> GGMTTMTVHTMGVHYKWQIPEVLRQQLWLAHNLREDLVSLQLAYDDDLKAIWSSYPDVAQAEDTMAAAEADAVALSERVKQARIEARSKKISTELTQQLRDAKKRLKDARQARRDAIAVVKDDAAERRKARSDQLAADQKALYGQYCRDGDLYWASFNTVLDHHKTAVKRIAAQRASGKPATLRHHRFDGSGTIAVQLQRQAGAPPRTPMVLADEAGKYRNVLHIPGWTDPDVWEQMTRSQCRQSGRVTVRMRCGSTDGQPQWIDLPVQVHRWLPADADITGAELVVTRVAGIYRAKLCVTARIGDTEPVTSGPTVALHLGWRSTEEGTAVATWRSDAPLDIPFGLRTVMRVDAAGTSGIIVVPATIERRLTRTENIASSRSLALDALRDKVVGWLSDNDAPTYRDAPLEAATVKQWKSPQRFASLAHAWKDNGTEISDILWAWFSLDRKQWAQQENGRRKALGHRDDLYRQIAAVISDQAGHVLVDDTSVAELSARAMERTELPTEVQQKIDRRRDHAAPGGLRASVVAAMTRDGVPVTIVAAADFTRTHSRCGHVNPADDRYLSNPVRCDGCGAMYDQDRSFVTLMLRAATAPSNP

A recent study demonstrated that the type V-M (formerly type V-U1, clade 2) Cas12m2 from Mycolicibacterium mucogenicum (hereafter referred to as Cas12m2 for simplicity) exhibits RNA-guided dsDNA interference activity. Cas12m2 associates with a single crRNA to recognize dsDNA targets containing a 5′-TTN-3′ PAM. Interestingly, Cas12m2 lacks target dsDNA-cleavage activity, probably due to the non-canonical His–Asp–Asp (HDD) catalytic residues in the RuvC domain, rather than the canonical, DNA-cleavable active site Asp–Glu–Asp (DED). Hence, instead of target cleavage, Cas12m2 interferes with invading MGEs through transcriptional silencing by strong DNA binding.

In state I, the target DNA forms a full R-loop containing a 17-bp heteroduplex, whereas, in state II, the target DNA only forms a 12-bp heteroduplex, and the displaced NTS is disordered. Nucleotides G1 to U17 in the crRNA and dA1 to dC17 in the target DNA strand (TS) form a 17-bp guide RNA–target DNA heteroduplex. Unexpectedly, nucleotides dG(−3) to dC(−1) in the TS do not form base pairs with G18 to C20 in the crRNA and instead rehybridize with dG18* to dC20* in the NTS, suggesting that the 17-bp guide RNA–target DNA heteroduplex represents the optimal length for Cas12m2-mediated DNA recognition (to differentiate between NTS and TS in this study, an asterisk is used to denote the NTS). By stark contrast, in the full R-loop, the REC2 domain is ordered and interacts with the sugar–phosphate backbone of the heteroduplex at the PAM-distal region. This structural rearrangement of the REC2 domain facilitates formation of the Arg-rich pocket between the REC1 and REC2 domains, allowing the binding of the displaced NTS. The displaced NTS passes through the groove formed by the REC1 and REC2 domains toward the groove formed by the RuvC and TNB domains. Notably, the central region of the negatively charged backbone of the NTS is bound to an Arg-rich pocket in the REC1 and REC2 domains and interacts extensively with Arg111, Arg112, Arg126 and Arg173. In the Cas12m2 structure, the nucleotides dG14* to dT17* in the NTS are clearly visible, and the phosphate group of dG16* is located at the RuvC active site formed by His317, Asp485 and Asp579 residues. At the position corresponding to magnesium ion (A) in other Cas12 enzymes, we observed a magnesium ion that was coordinated by His317 and Asp579, whereas no density corresponding to magnesium ion (B) was observed. Nonetheless, His317 and Asp579 are bound to the NTS via magnesium ion coordination, and His317 is stabilized by hydrogen bonding with Asp485, suggesting that the HDD motif plays a crucial role in target DNA binding, rather than target DNA cleavage.> ANLNGTLMQYFEWYMPNDGQHWKRLQNDSAYLAEHGITAVWIPPAYKGTSQ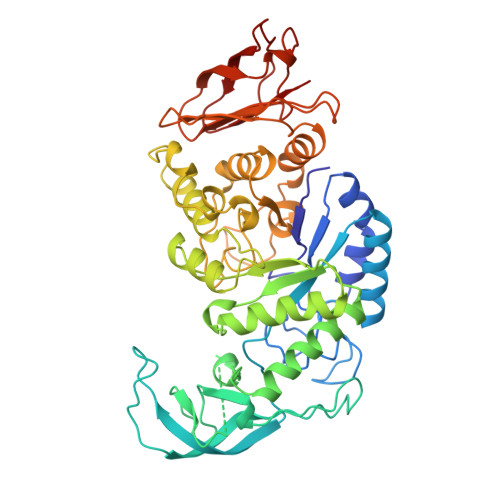ADVGYGAYDLYDLGEFHQKGTVRTKYGTKGELQSAIKSLHSRDINVYGDVVINHKGGADATEDVTAVEVDPADRNRVISGEHLIKAWTHFHFPGRGSTYSDFKWHWYHFDGTDWDESRKLNRIYKFQGKAWDWEVSNENGNYDYLMYADIDYDHPDVAAEIKRWGTWYANELQLDGFRLDAVKHIKFSFLRDWVNHVREKTGKEMFTVAEYWQNDLGALENYLNKTNFNHSVFDVPLHYQFHAASTQGGGYDMRKLLNSTVVSKHPLKAVTFVDNHDTQPGQSLESTVQTWFKPLAYAFILTRESGYPQVFYGDMYGTKGDSQREIPALKHKIEPILKARKQYAYGAQHDYFDHHDIVGWTREGDSSVANSGLAALITDGPGGAKRMYVGRQNAGETWHDITGNRSEPVVINSEGWGEFHVNGGSVSIYVQR3'-DEOXY-3'-ACETAMIDO-URIDINE 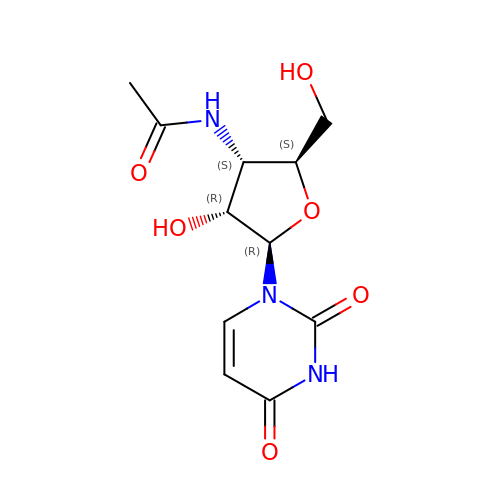| C11 H15 N3 O6 | BUUSLPRPRSICHU-JLRHVRHOSA-N> GPERTSIAVHALMGLPTGQPANGTKLDSIGLPKVDGMSFTLYR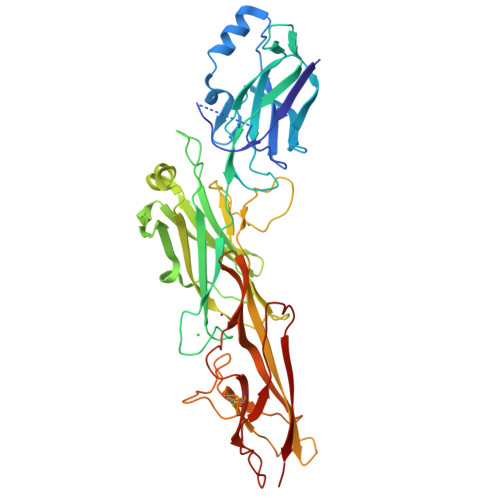VNEIDLTTQAGWDAASKIKLEELYTNGHPTDKVTKVATKKTEGGVAKFDNLTPALYLVVQELNGAEAVVRSQPFLVAAPQTNPTGDGWLQDVHVYPKHQALSEPVKTAVDPDATQPGFSVGENVKYRVATKIPEIASNTKFEGFTVADKLPAELGKPDTNKITVTLGGKPINSTDVSVQTYQVGDRTVLSVQLAGATLQSLDQHKDQELVVEFEAPVTKQPENGQLDNQAWVLPSNPTAQWDPEESGDAALRGMPSSRVSSKFGQITIEKSFDGNTPGADRTATFQLHRCEADGSLVKSDPPISLDGKQEFVTGQDGKAVLSGIHLGTLQLESNVMKYTDAWAGKGTEFCLVETATASGYELLPKPVIVKLEANESTNVLVEQKVKIDNKKKN> MRCLALDIGGTKIAAAIVKNEIEQRQQIHTPRENVVEGMHQALGKLLADYEGQFDYVAVASTGIINNGILSALNPKNLGGLAEFPLKASIAKHTDKPIGLLNDAQAATYAEYQL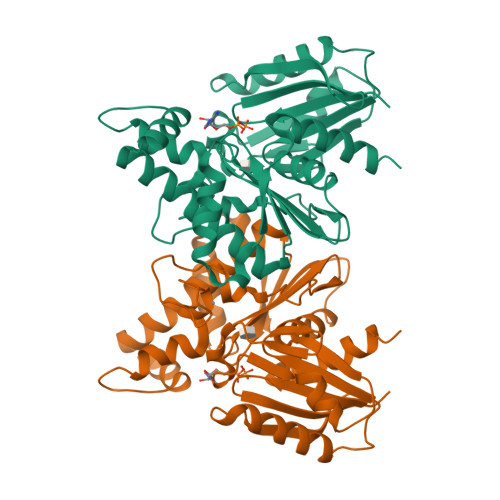QNFEQVSNFVFITVSTGVGGGIVLNQILQTGSRGIAGHIGHTLADPNGAICGCGRRGCVEAIASGRAIEAVSSQWEDPCDPKEVFERFRKNDEKATALVERSAKAIANLIADLVISLDIQKIAIGGSVGLAEGYLSLVEKYLQDFPSIYCCEIETAKFGQDAGLIGAAYWVKDVLL>[3x]NGHLQHHPPMPPHPGHYWPVHNELAFQPPISNHPAPEYWCSIAYFEMDVQVGET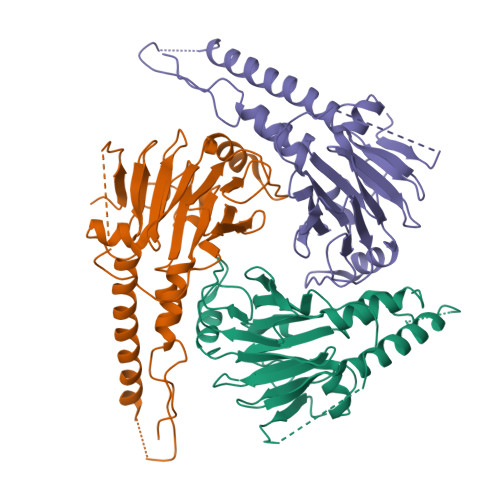FKVPSSCPIVTVDGYVDPSGGDRFCLGQLSNVHRTEAIERARLHIGKGVQLECKGEGDVWVRCLSDHAVFVQSYYLDREAGRAPGDAVHKIYPSAYIKVFDLRQCHRQMQQQAATAQAAAAAQAAAVAGNIPGPGSVGGIAPAISLSAAAGIGVDDLRRLCILRMSFVKGWGPDYPSQSIKETPCWIEIHLHRALQLLDEVLHTMPIADPQPLD> GGDQRFGDLVFRQLAPNVWQHTSYLDMPGFGAVASNGLIVRDGGRVLVVDTAWTDDQTAQILNWIKQEINLPVALAVVTHAHQDKMGGMDALHAAGIATYANALSNQLAPQEGLVAAQHSLTFAANGWVEPATAPNFGPLKVFYPGPGHTSDNITVGIDGTDIAFGGCLIKDSKAKSLGNLGDADTEHYAASARAFGAAFPKASMIVMSHSAPDSRAAITHTARMADKLR

The bacterial metallo-β-lactamases (MBLs) catalyze the inactivation of β-lactam antibiotics. Class B members, known as the metallo-β-lactamases (MBLs), are structurally distinct from the Class A, C, and D enzymes, require one or two zinc ions for catalytic activity, and are not inhibited by currently approved therapeutics. One variant of significance is NDM-4, first identified in 2012 (17). Although it differs from NDM-1 by a single amino acid substitution, namely M154L, it demonstrates increased enzymatic activity against the carbapenems and several cephalosporins.

Crystals of the NDM-4/Compound 1 complex were obtained from poly(ethylene glycol) 3350 solutions at pH 6.0 and contained one molecule per asymmetric unit. The model was refined to an overall R-factor of 20.3% at 1.3 Å resolution. Compound 1 functions as a bidentate ligand to Zn2, which is also surrounded by the side chains of Asp 124, Cys 208, and His 250 and the bridging solvent in an octahedral coordination sphere. The bond distances between Zn2 and the sulfur and oxygen atoms of Compound 1 are 2.5 Å and 2.0 Å, respectively. The coordination geometry around Zn1 remains tetrahedral with the side chains of His 120, His 122, and His 189, and the bridging solvent serving as ligands. Both the side chain of Lys 211 and backbone amide nitrogen of Asn 220 serve to anchor the carboxylate moiety of Compound 1 into the active site. In addition to the difference in coordination geometry to the binuclear metal center, the side chain of Asn 220 swings toward the active site upon Compound 1 binding. Within experimental error, the distance between Zn1 and Zn2 when Compound 1 binds remains the same as observed in the apoenzyme model (∼3.6 Å). In the NDM-4/Compound 1 complex, the bridging water is within 1.9 Å and 2.0 Å from Zn1 and Zn2, respectively. Our results demonstrate that Compound 1, an inhibitor directed against NDM-4, demonstrates a unique binding mode, whereby it forms a bidentate interaction with Zn2 in an octahedral coordination sphere.>[8x]GDVAAGASVFSANCAACHMGGRNVIVANKT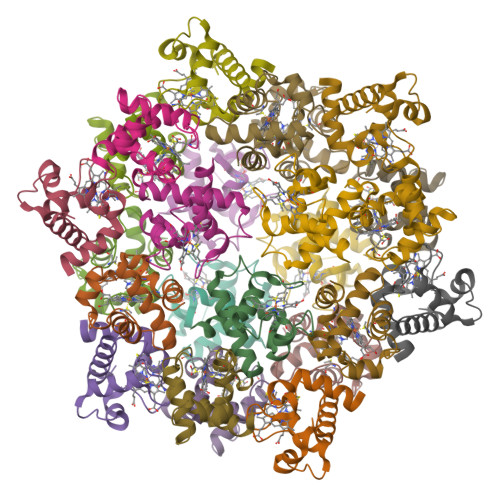LSKSDLAKYLKGFDDDAVAAVAYQVTNGKNAMPGFNGRLSPKQIEDVAAYVVDQAEKGW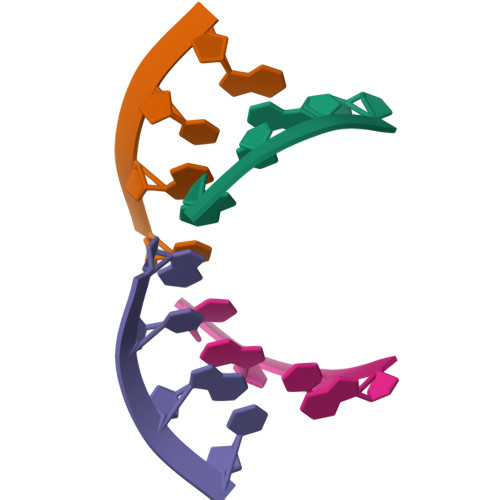>[2x]CGCG;>[2x]GCGC Protein modifications by ubiquitin and Ubl (ubiquitin-like) proteins are involved in the regulation of most cellular pathways including cell cycle progression, transcription, DNA repair and stress responses, and their misregulation is implicated in cancer and aging. Both ubiquitin and SUMO (small ubiquitin-related modifier) can form substrate-attached chains, in which one unit of the respective modifier is attached to a lysine residue of another. SUMO is recognized by short SIMs (SUMO-interaction motifs) that have specific consensus sequences and bind with medium to low affinity with dissociation constants in the range 1–100 μM. Upon binding to a hydrophobic groove present in SUMO1 as well as SUMO2/3, the unstructured SIMs adopt a β-strand conformation that forms a parallel (SIMa and SIMb) or antiparallel (SIMr) β-sheet together with the β2-strand of SUMO. STUbLs are conserved in all eukaryotes, and the mammalian STUbL RNF4 (RING finger protein 4) complements deletions of STUbL genes in yeast.

In order to analyse the contribution of the four putative SIMs in RNF4 to the binding of SUMOylated substrates, we tested the interaction of full-length RNF4 and of a construct comprising the entire N-terminal part of RNF4 upstream of the RING domain (subsequently referred to as ‘SIM domain’) with mono-SUMO1 and mono-SUMO2 and with linear SUMO–SUMO fusion proteins of variable length. These SUMO fusion proteins lacked the N-terminal 11 residues of each SUMO, thus retaining the natural distance as it occurs within a natural Lys11-linked SUMO chain. The last residue at the C-terminus of the first SUMO monomer in the proposed di-SUMO2 and the first N-terminal residue of the second SUMO monomer that are resolved in the structure are 14.1 Å (1 Å=0.1 nm) apart. The linker region in between comprises 11 residues and is not resolved, indicating that it is structurally flexible. The residues of this stretch can easily cover the distance of 14.1 Å in an extended form. Therefore a SUMO chain in solution is expected to be able to adopt multiple conformations to interact with the SIMs in unstructured regions of SUMO-binding proteins. Importantly, we found almost no difference in binding of the linear di-SUMO fusions compared with the binding affinity of ‘native’ Lys11-linked di-SUMO2 chains (KD=11 μM). This validates that linear SUMO fusions are a suitable model for poly-SUMOs and that the SIM domain of RNF4 recognizes the SUMO chain only via the established SUMO–SIM interaction and not by additional binding to the branching point at Lys11. The interaction of the SIM domain with linear di-SUMOs was stronger, with similar dissociation constants (KD) of 17 μM for di-SUMO1 and 14 μM for di-SUMO2. Elongation of the SUMO chain to four moieties, however, resulted in a significant increase in affinity with a KD value of 4.3 μM for tetra-SUMO1 and 1.6 μM for tetra-SUMO2.

> GSTENNDHINLKVAGQDGSVVQFKIKRHTPLSKLMKAYCERQGLSMRQIRFRFDGQPINETDTPAQLEMEDEDTIDVFQQQTGGRSTENNDHINLKVAGQDGSVVQFKIKRHTPLSKLMKAYCERQGLSMRQIRFRFDGQPINETDTPAQLEMEDEDTIDVFQQQTGG> UUUUUAA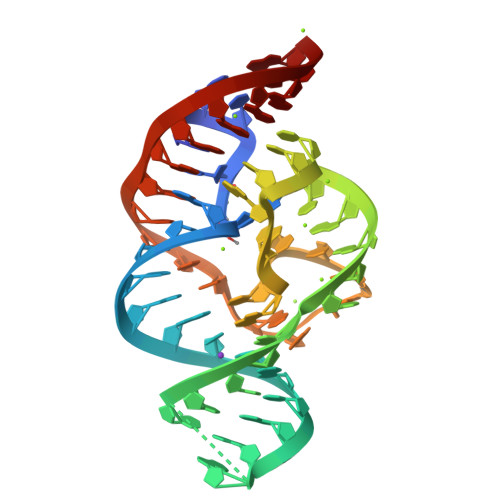UGAAGCCACAGGCUGUGAGGGUCCUAAGCCCCUAAUUCAGAAGGGAA>TPLGPASSLPQSFLLKCLEQVRKIQGDGAALQEKLCATYKLCHPEELVLLGHSLGIPWAPLSSCPSQALQLAGCLSQLHSGLFLYQGLLQALEGISPELGPTLDTLQLDVADFATTIWQQMEELGMAPALQPTQGAMPAFASAFQRRAGGVLVASHLQSFLEVSYRVLRH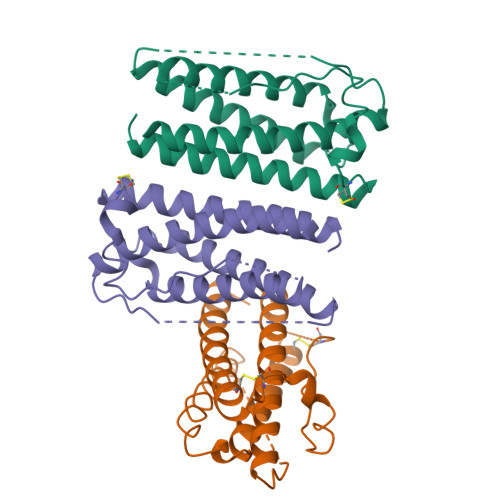LAQP[3x]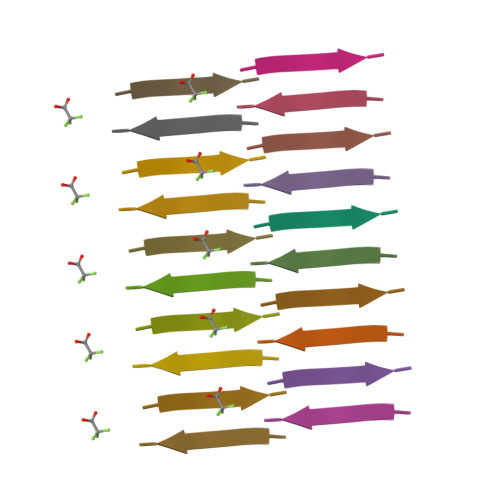>[2x]IYKVEI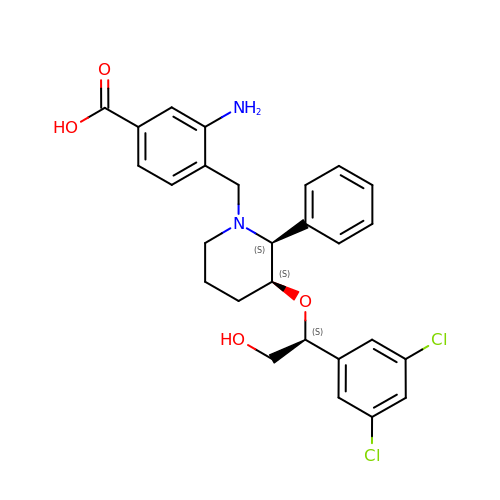3-amino-4-({(2S,3S)-3-[(1S)-1-(3,5-dichlorophenyl)-2-hydroxyethoxy]-2-phenylpiperidin-1-yl}methyl)benzoic acid | C27 H28 Cl2 N2 O4 | WIHIMICVVOCQNM-NXCFDTQHSA-N> MSVETPSALADSSPHTAPGSAGRSLELGAADIQDLESFEAGRGALPARAYLQSDAPRLSLNGEWQFRLSPGSRVAPDDGW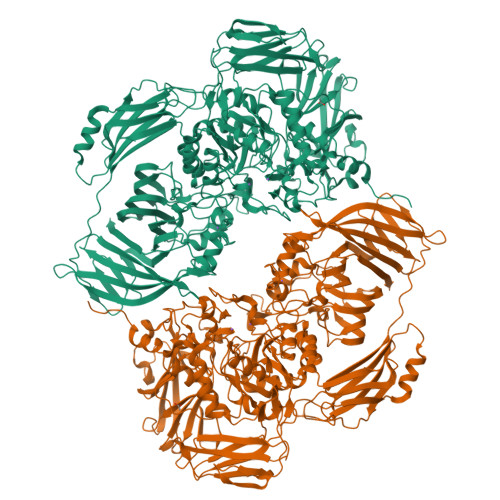QLGEALNGFESLPVPSSWPMHGHGAPAYTNVQFPFAVEPPHVPEANPIGDHLVVFEAGPEFFPHALLRFDGIESAGTVWLNGVELGTTRGSRLAHEFDVSGILEQGENTLAVRVAQFSAASYVEDQDMWWLPGIFRDVTLQARPAAGIDDVFVHAGYDHITGEGILKVEASRGGQAIDAVVRVPELALELAAGTEVRVPAVEPWSAEVPKLYEAAVSAAGESVALQIGFRSIAIEDAQFKVNGRRILLRGVNRHEHHPRLGRVVPRDVVEAELRLMKQHNINAIRTSHYPPHPQFLALADQLGFYVVLECDLETHGFESAGWAQNPSDDPQWEDALVDRMRRTVERDKNHASVVMWSLGNEAGTGRNLAAMSRWTKDRDPSRPIHYEGDWSSEHVDVYSRMYASQAETALIGQGIEPALNDAALDARRRAMPFVLCQYVHAMGNGPGGMSEYQALFEKYPRLMGGFVWEWLEHGITVSTADGVDHYGYGGDFGEEVHDGNFVTDGLVDADRRPRPGLLDFKKVIEPLRIDVARDWTGFTLRNGQDFADTSAFSFRYEVEADGGALDGGTVDVAPVAPQSETVVELPGSVAALAAGLSDGRPAVLTVRAVLGADSAWADAGHEVAWGQSVREPGAPVPPAPVEPVQVQDSELTLGPVVFSRATGMPTSIGGVPVEKLGLTLWWAPTDNDLGREWGGADERPLATQWKDAGLNRLHTRLLGISANPGQDGGETLTVRTRVSAADKQYGVLVDYTWSTDGETVGLRTQVRRDGTWVNRGFEVEWARIGLEFVLGEETELVSWFGQGPHQSYPDTGQGARAGWFSLPLAKMDVEYVRPQECGARSGSRSAALQLGGRTLEICGDPFALTVRPYSQDVLDAAAHRPDLKADGRTYLYVDHALRGVGTAACGPGVLEQYRLKPRDADFILTLKVRS>[8x]MTNETSDRPLVHFTPNKGWMNDPNGLWYDEKDAKWHLYFQYNPNDTVWGTPLFWGHATSDDLTNWEDQPIAIAPKRNDSGAFSGSMVVDYNNTSGFFNDTIDPRQRCVAIWTYNTPESEEQYISYSLDGGYTFTEYQKNPVLAANSTQFRDPKVFWYEPSQKWIMTAAKSQDYKIEIYSSDDLKSWKL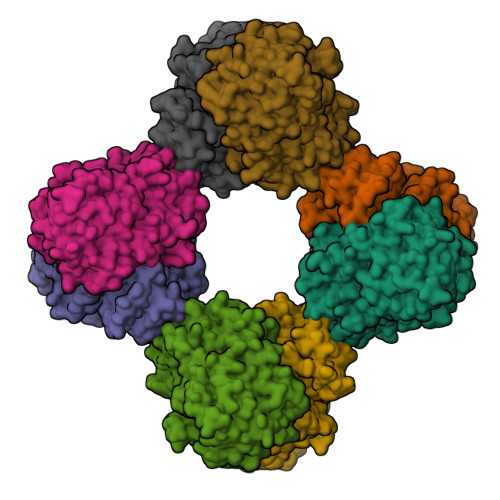ESAFANEGFLGYQYECPGLIEVPTEQDPSKSYWVMFISINPGAPAGGSFNQYFVGSFNGTHFEAFDNQSRVVDFGKDYYALQTFFNTDPTYGSALGIAWASNWEYSAFVPTNPWRSSMSLVRKFSLNTEYQANPETELINLKAEPILNISNAGPWSRFATNTTLTKANSYNVDLSNSTGTLEFELVYAVNTTQTISKSVFADLSLWFKGLEDPEEYLRMGFEVSASSFFLDRGNSKVKFVKENPYFTNRMSVNNQPFKSENDLSYYKVYGLLDQNILELYFNDGDVVSTNTYFMTTGNALGSVNMTTGVDNLFYIDKFQVREVK> SGIVQQQNNLLRAIEAQQHLLQATVWGIKQLQARSGGRGGWMEWDREIN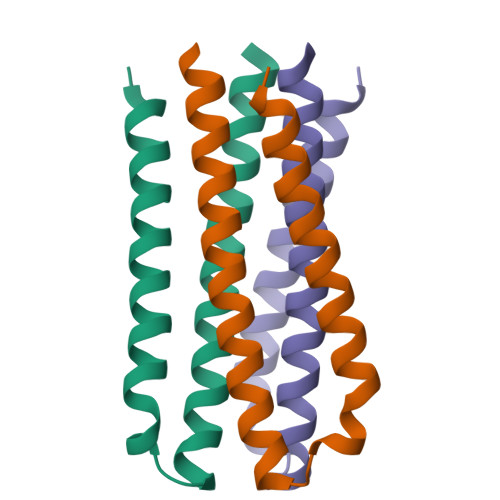NYTSLIHSLIEESQNQQEK[[(2~{R},3~{S},4~{R},5~{R})-5-[2,6-bis(oxidanylidene)-3~{H}-purin-9-yl]-3,4-bis(oxidanyl)oxolan-2-yl]methoxy-oxidanyl-phosphoryl] 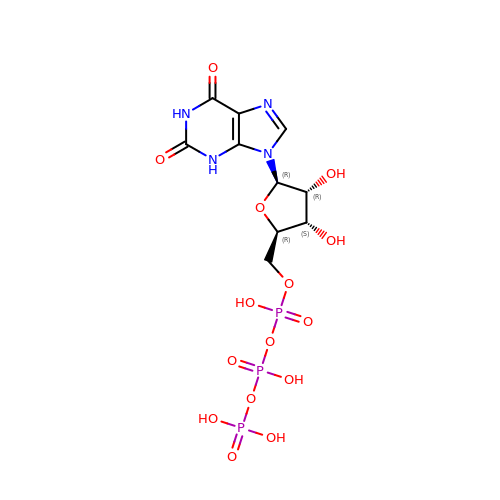phosphono hydrogen phosphate | C10 H15 N4 O15 P3 | CAEFEWVYEZABLA-UUOKFMHZSA-N> MGSSHHHHHHSQDPMNRPSFNEAWLAFRKVNHSVADVGSIIGGNVGKNITGGYFQNACPIRMSYVLNATGFPIARNSPYAKVSGADNKFYIYRVNDMIDYLTHTMG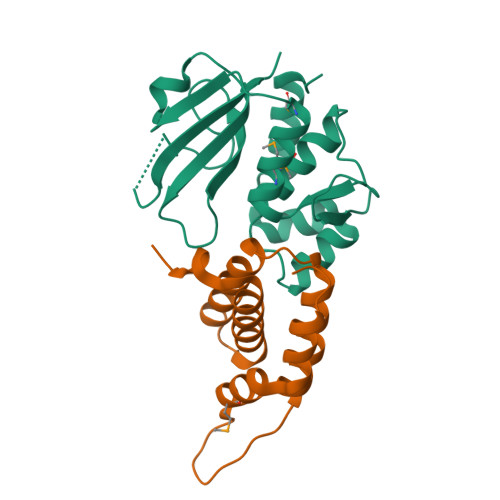KPDLIVNNPKQSDFIGKKGIIVVKGHGWSNARGHVTLWNGSICSDQCHLLNDPDNGPFVPEVGTLWILP;> MFAQEALTTQYSQSELLKNWALSHCLALVYKDDVVKNDARATASAYLEYGKQSVEIYHEIDEIAKKYSGLKYNGSISSDFNTMKCIDFIHDRELNELIKRRVEK Sugars and other sweet-tasting compounds are detected by the sweet taste receptor, a member of the class C GPCR family. The sweet receptor is a heterodimer composed of TAS1R2 and TAS1R3,3,4 two type 1 taste receptor family members that share the distinctive architecture of class C GPCRs: a large extracellular Venus flytrap (VFT) domain, responsible for ligand recognition; a cysteine-rich domain (CRD); and a seven-transmembrane (7TM) domain that mediates G protein coupling. To address this gap, here we present cryo-electron microscopy (cryo-EM) structures of the sweet receptor in the inactive, unliganded state, as well as in the activated, sucralose- and advantame-bound states. Unlike other class C GPCRs, such as mGluR, CaSR and GABAB receptors, where agonists stabilize inter-subunit VFT interactions to promote activation, the sweet receptor is activated by the rearrangement of a TAS1R2 VFT loop, which destabilizes interactions between the lower VFT lobes and the VFT–CRD interfaces.

In the presence of sweeteners, the human/mouse sweet receptor adopts two distinct conformations, which we refer to as compact and loose. In the compact conformation, the VFT LB2s remain packed; in the loose conformation, LB2s of the two subunits disengage. Advantame also yields well-defined ligand density in the TAS1R2 VFT pocket of both human/mouse and human/human receptors. Advantame adopts a bent, arched pose within the clamshell cleft, with its Phe/Asp dipeptide core and vanillyl aromatic ring extending across the clamshell. Advantame engages TAS1R2 Ser144 through polar contacts, and its hydroxyl and amine groups form hydrogen bonds with conserved Asp142, Asp278, and Glu302. Although its interactions with TAS1R2 differ from those of sucralose, advantame elicits a comparable conformational change: the bottom of LB2 lifts by up to 8 Å, and the clamshell opening decreases from 112° (apo) to 104° (compact) and 103° (loose). The closure of the TAS1R2 VFT clamshell induced by sweetener binding leads to the formation of salt bridges between LB1 Lys65 and LB2 Asp278, which are brought into proximity in the compact state and engage further to form stable interactions in the loose state. By contrast, in the compact state, the inter-lobe interface remains largely preserved relative to the apo state, with the distance between the LB2s changing by only 0.7 Å. First, agonist binding induces clamshell closure in TAS1R2, accompanied by a stabilizing salt bridge that defines the compact state.

> AENSDFYLPGDYLLGGLFSLHANMKGIVHLNFLQVPMCKEYEVKVIGYNLMQAMRFAVEEINNDSSLLPGVLLGYEIVDVCYISNNVQPVLYFLAHEDNLLPIQEDYSNYSSRVVAVIGPDNSESVMTVANFLSLFLLPQITYSAISDELRDKVRFPALLRTTPSADHHIEAMVQLMLHFRWNWIIVLVSNDTYGRDNGQLLGERVARRGICIAFQETLPTLQPNQNMTSEERQRLVTIVDKLQQSTARVVVVFSPDLTLYHFFNEVLRQNFTGAVWIASESWAIDPVLHNLTELRHLGTFLGITIQSVPIPGFSEFREWGPQAGPPPLSRTSQSYTCNQECDNCLNATLSFNTILRLSGERVVYSVYSAVYAVAHALHSLLGCDKSTCTKRVVYPWQLLEEIWKVNFTLLDHQIFFDPQGDVALHLEIVQWQWDRSQNPFQSVASYYPLQRQLKNIQDISWHTINNTIPMSMCSKRCQSGQKKKPVGIHVCCFECIDCLPGTFLNHTEDEYECQACPNNEWSYQSETSCFKRQLVFLEWHEAPTIAVALLAALGFLSTLAILVIFWRHFQTPIVRSAGGPMCFLMLTLLLVAYMVVPVYVGPPKVSTCLCRQALFPLCFTICISCIAVRSFQIVCAFKMASRFPRAYSYWVRYQGPYVSMAFITVLKMVIVVIGMLATGLSPTTRTDPDDPKITIVSCNPNYRNSLLFNTSLDLLLSVVGFSFAYMGKELPTNYNEAKFITLSMTFYFTSSVSLCTFMSAYSGVLVTIVDLLVTVLNLLAISLGYFGPKCYMILFYPERNTPAYFNSMIQGYTMRRD;> ASLCLSQQFKAQGDYILGGLFPLGSTEEATLNQRTQPNSIPCNRFSPLGLFLAMAMKMAVEEINNGSALLPGLRLGYDLFDTCSEPVVTMKSSLMFLAKVGSQSIAAYCNYTQYQPRVLAVIGPHSSELALITGKFFSFFLMPQVSYSASMDRLSDRETFPSFFRTVPSDRVQLQAVVTLLQNFSWNWVAALGSDDDYGREGLSIFSSLANARGICIAHEGLVPQHDTSGQQLGKVLDVLRQVNQSKVQVVVLFASARAVYSLFSYSIHHGLSPKVWVASESWLTSDLVMTLPNIARVGTVLGFLQRGALLPEFSHYVETHLALAADPAFCASLNAELDLEEHVMGQRCPRCDDIMLQNLSSGLLQNLSAGQLHHQIFATYAAVYSVAQALHNTLQCNVSHCHVSEHVLPWQLLENMYNMSFHARDLTLQFDAEGNVDMEYDLKMWVWQSPTPVLHTVGTFNGTLQLQQSKMYWPGNQVPVSQCSRQCKDGQVRRVKGFHSCCYDCVDCKAGSYRKHPDDFTCTPCNQDQWSPEKSTACLPRRPKFLAWGEPVVLSLLLLLCLVLGLALAALGLSVHHWDSPLVQASGGSQFCFGLICLGLFCLSVLLFPGRPSSASCLAQQPMAHLPLTGCLSTLFLQAAETFVESELPLSWANWLCSYLRGLWAWLVVLLATFVEAALCAWYLIAFPPEVVTDWSVLPTEVLEHCHVRSWVSLGLVHITNAMLAFLCFLGTFLVQSQPGRYNRARGLTFAMLAYFITWVSFVPLLANVQVAYQPAVQMGAILVCALGILVTFHLPKCYVLLWLPKLNTQEFFLGRNAKKAADENSGGGEAAQGHNE>[2x]GLTYSQTMELKDSMLQLDPNAKTWIDIEGRPEDPVEIAIYQPNNGQYIHFYREPTDIK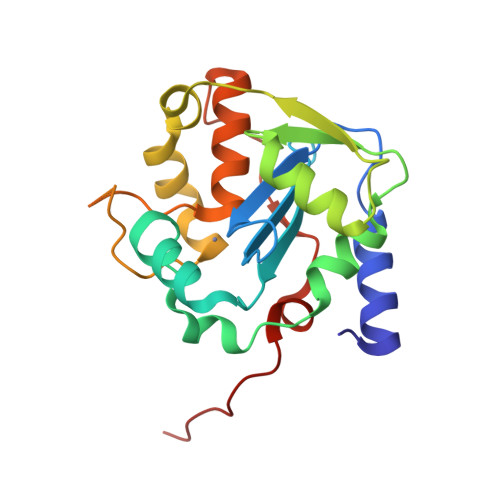QFKQDSKHSHGIDIQDLFSVQPGLTSAVIESLPKNMVLSCQGADDIRKLLDSQNRRDIKLIDVSMQKDDARKFEDKIWDEYKHLCRMHTGIVTQKKKRGGKEEVTPHCALLDCLMFEAAVIGSPQIPTPRPVLSRDLVFRTGPPRVVL>[4x]MAETAPLRVQLIAKTDFLAPPDVPWTTDADGGPALVEFAGRACYQSWSKPNPKTATNAGYLRHIMDVGHFSVLEHASVSFYITGISRSCTHELIRHRHFSYSQLSQRYVPEKDSRVVVPPGMEDDADLRHILTEAADAARATYSELLAKLEAKFADQPNAILRRKQARQAARAVMPNATETRIVVTGNYRAWRHFIAMRASEHADVEIRRLAIECLRQLAAV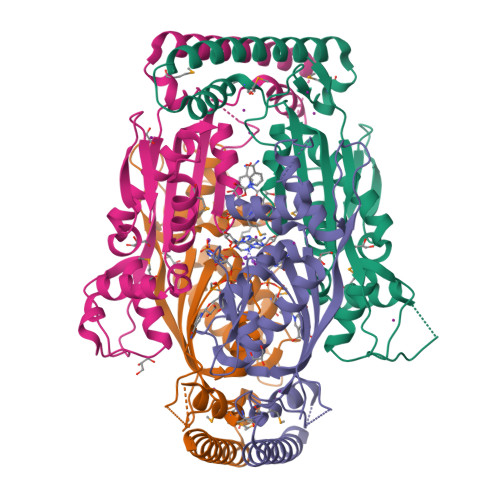APAVFADFEVTTLADGTEVATSPLATEALEHHHHHH> MKVLQEPTCVSDYMSISTCEWKMNGPTNCSTELRLLYQLVFLLSEAHTCIPENNGGAGCVCHLLMDDVVSADNYTLDLWAGQQLLWKGSFKPSE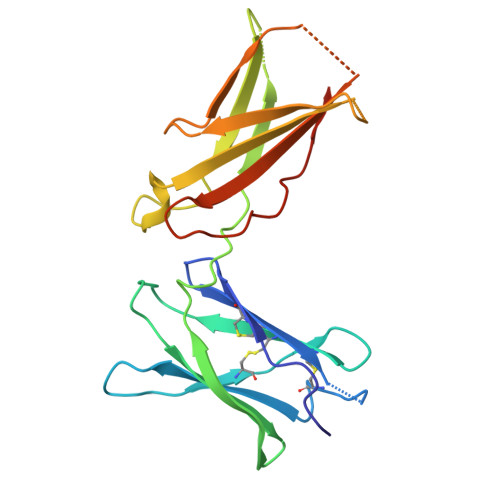HVKPRAPGNLTVHTNVSDTLLLTWSNPYPPDNYLYNHLTYAVNIWSENDPADFRIYNVTYLEPSLRIAASTLKSGISYRARVRAWAQCYNTTWSEWSPSTKWHNSYREP> MSLKVVSVDTLCCDAGWRNYHFVKLTTDEGIVGWSEFDEGFGSPGVTAVIEQLGKRLVGASVMEHERFFAEAYCLTRPATGGVVSEGIGAIENALLDAKAKTLNVPCYELLGGKLRDRVPVYWSHCPTWRINHP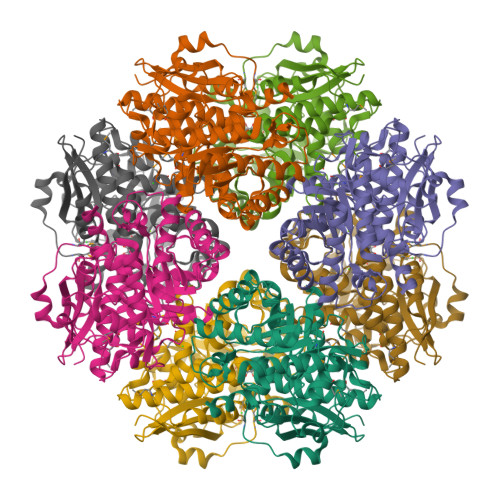KFFGPPVTDLDGVKRTAEEARERQFRAIKTNIFIHDDGPLHAWRPGFAVPFQPALNVDRKVLRNLRAHLEALRDGAGPDVEILLDLNFNAKPEGYLKILRELADFDLFWVEIDSYSPQGLAYVRNHSPHPISSCETLFGIREFKPFFDANAVDVAIVDTIWNGVWQSMKIAAFADAHDINVAPHNFYGHLCTMINANFAAAVPNLRIMETDIDRLAWEDELFTHAPEYQNGELIIPDRPGWGTDPVEEAILAHPPKVMGGLLQYKRSEGHHHHHH>[7x]HPSEPGVVSYAVLGKGSVGNIVGAPMGWEAVFTRPFQAFWVELPACNNWVDIGLPEVYDDPDLAS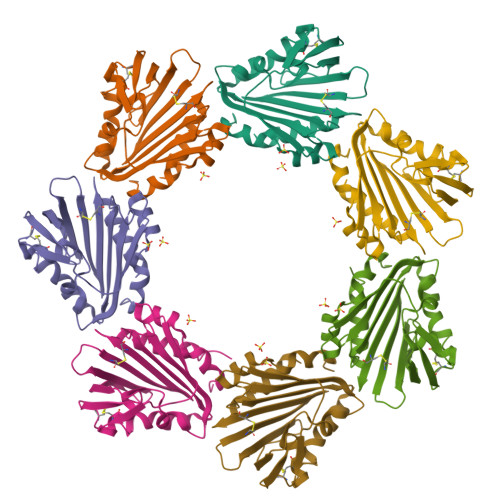FNGATTQTSATDQTHLVKQAVGVFASNDAADRAFHRVVDRTVGCSGQTTAIHLDDGTTQVWSFAGGPSTGTDEAWTKQEAGTDRRCFVQTRLRENVLLQAKVCQSGNAGPAVNVLAGAMQNTLGKLAAALEHHHHHH>[2x]ETGIGQRIVCLVLDKSGSMATGNRLNRLNQAGQLFLLQTVELGSWVGMVTFDSAAHVQSELIQINSGSDRD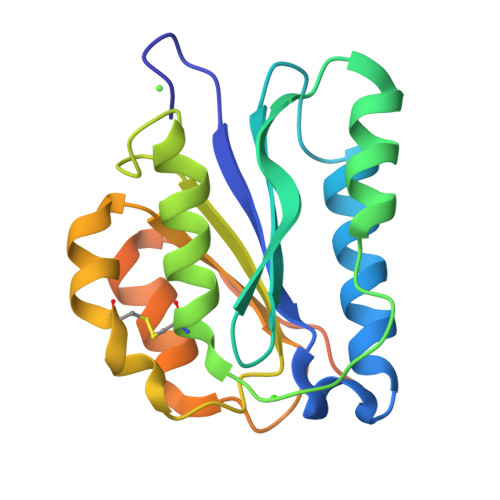TLAKRLPAAASGGTSICSGLRSAFTVIRKKYPTDGSEIVLLTDGEDNTISGCFNEVKQSGAIIHTVALGPSAAQELEELSKMTGGLQTYASDQVQNNGLIDAFGALSGTKHHHHHH>[2x]MGRDPNSSSVDKLAAALEHHHHHHMSAVASHVVPPRSKLDSILSSGLEHNIDHDPLEVWDKGVFLNELLKQGIALSTNENGTLDGELVADEGLKKGSYKGTRLALTEIYSILEDAAVSHF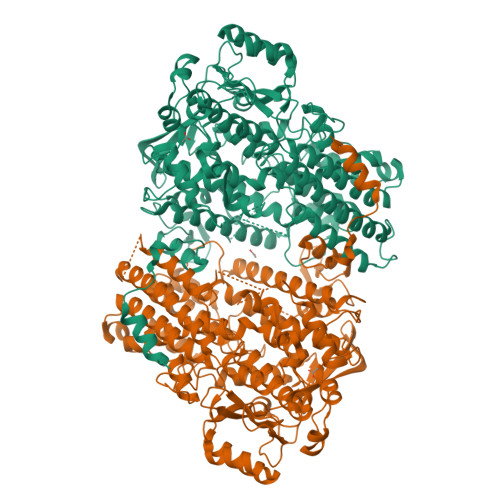DKRGYEPIFPVKRELDLKKRIYQWSDGTDGYPPHLKVDGNDEANLPADERQSKPGSARSEGVGQIFDMQETAFVSKIAQAVSFIIPKDIDHENTPYKGPTLADVEKFNKAQFPKTDGDASNQDNLNKAADIMKGRNIGEYDDWYSDARFAQQHFSGVNPSTIETASQDKIKEYISEAQKQGLDKVKAILEDGKDILIQDYSYFREATGATNEQIFQNTVYELKGTTPTGKTTSRYAAASVVIFQLHEDGRLHPLAITLDYKGSLDNSITIFNRRLSPDDTCDIAEKEDWPWRYAKTVAQTADWARHEVATHLVDTHMIEEAIIVATNRIIPEGELLYEILSPHWFRTLSLNAAARKLLVPGVIARIAGFGPTSPSLDFKGNNAFKLIDWSYKNFNFQDKYIPNDLKKRGFDIKGDKSGKYKNYPYANDMYLLWGIIRNFVKTVIESQYTSDHVVQKDPYIGGWCKEIQTNGQIPTFPTITTVEQLIDAVTMCIHTASPQHTAVNYLQDYYYSFVPAKPPALCTPLPQDLSALQGYTEKDLTAALPIGTEDMKWKDWLLAAQLPELLSYKVQQDYNLITYAKSLYNVNKNRTITENTKFNCKTIKKAAADFYSHLKSAGVEFENYSKGQTAGTVEYPVLQPETTAISILI>[4x]NDELIKLEKEPGQW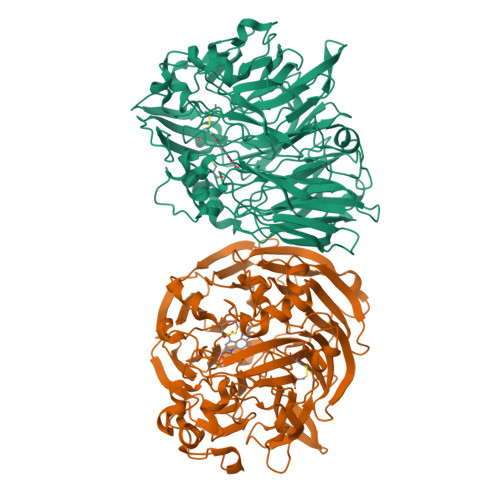VMQNKNYANTRYSELNQINTKNVSRLRLAWSFSTGALRGHEGGPLVVGTTMYVHSAYPNHVYALDLTQKPYAIKWQYTPVQNSQAVAVACCDVVNRGLAYANGKIFMTTLDGQIIALDANTGKELWKMKHADVTKGETITGAPLVVKDKVLVGVSGGEFGVRGRVGAYDINTGNRVWLAYSQGPDEEVLLDSDFNKEFPQHGGPGDGTKTWPGEQWKLGGGTTWGWYSYDPALDLFYYGTSNPGTWNAEQRKGGDNKWSCTIFARRPDTGKARWAYQMTPWDSWDYDGVNEMILPDLTVKGKKTPCLVHFDRNGFGYVLDRRTGQLIEAQPFVYVNWAKEISKENDRPVEIPEKRTKQGVDTKGICPNSMGGKDQQPAAFSPQTGLFYVPTNNMCMNYEGVEATYTAGAPYVGANVLMYSGHEGKDDYYGAFICYDALKGKRVWEIHEHFPVWSGPVVTAGGLAFYGTMDGWFKAVDIKTGKVLWQQKLGSGIIGNPITFLGPDKKQYVAVYSGVGGWFGIAVAQNLPPDDPYAGLGAVGVAYQAGLPKATTVGGELYVFALE Here, we choose lipase B from Candida antarctica (CALB), as the model enzyme, in which Asp187-His224-Ser105 is the catalytically active triad. Lipases function according to the classical Ser-His-Asp catalytic triad mechanism. In the present study we propose that the Ser → Cys conversion in lipases may lead to high activity by accurate manipulation of the local environment surrounding the hybrid Cys-His-Asp triad, enabled by laboratory evolution. We succeed in evolving cysteine-CALB mutants that are even more active than WT CALB.

Surprisingly, Cys105 in variant QW4 appeared to be oxidized to the respective sulfinic acid. When purification and crystallization were performed in a glove box, Cys105 in the crystal structure was in the normal (reduced) state. An extremely high catalytic efficiency was observed for the purified variant QW4 (kcat/Km = 5920 s−1M−1), with kcat increased by 6 folds and catalytic efficiency (kcat/Km) increased by 40 folds compared with WT. Interestingly, the nucleophile exchange (S105C) in QW4 results in a conformational change of helix 277–288, compared with QW10 or WT. While the helixes of QW10 and WT CALB are well superimposable, the helix section P280-Y282 of QW4 is deformed and shifted toward the active site, with an additional H-bond between Y281 and E188 formed. The interactions with Y281 and E188 in QW4 further positions the substrate in the catalytic pocket of the enzyme. In striking contrast, the potential energy surface scan for QW4 disclosed that the acylation reaction follows a two-step mechanism involving a HisH+/CysS− ion pair, in which the proton is first transferred from the thiol group of C105 to H224, and then the negatively charged thiolate anion acts as a nucleophile, attacking the carbon of ester bond of the substrate to yield the tetrahedral intermediate. The first step, i.e., the proton transfer from SH of C105 to H224 is the rate determining step with an activation barrier of 13.95 kcal/mol, and then the thiolate anion attacks the carbonyl of the substrate rapidly with a low barrier of 6.2 kcal/mol. However, optimization of the point which is closest to a transition state corresponding to the concerted mechanism always led to the Cys105−/His224+ zwitterioinic pair, indicating the concerted mechanism is not preferred for variant QW4. The high catalytic efficiency of QW4 is attributed to its optimal binding properties, as well as the relatively low reaction barrier in the rate-determining step.

>GAMALPSGSDPAFSQPKSVLDAGLTCQGASPSSVSKPILLVPGTGTTGPQSFDSNWIPLSAQLGYTPCWISPPPFMLNDTQVNTEYMVNAITTLYAGSGNNKLPVLTVCQGGLVAQWGLTFFPSIRSKVDRLMAFAPDYKGTVLAGPLDALAGSAPSVWQQTTGSALTTALRNAGGLTQIVPTTNLYSATDEIVQPQVSNSPLDSSYLFNGKNVQAQAVCGPLFVIDHAGSLTSQFSYVVGRSALRSTTGQARSADYGITDCNPLPANDLTPEQKVAAAALLAPYYAAIVAGPKQNCEPDLMPYARPFAVGKRTCSGIVTP[2x]>FPTDDDDKIVGGYTCAANSIPYQVSLNSGSHFCGGSLINSQWVVSAAHCYKSRIQVRLGEHNIDVLEGNEQFINAAKIITHPNFNGNTLDNDIMLIKLSSPATLNSRVATVSLPRSCAAAGTECLISGWGNTKSSGSSYPSLLQCLKAPVLSDSSCKSSYPGQITGNMICVGFLEGGKDSCQGDSGGPV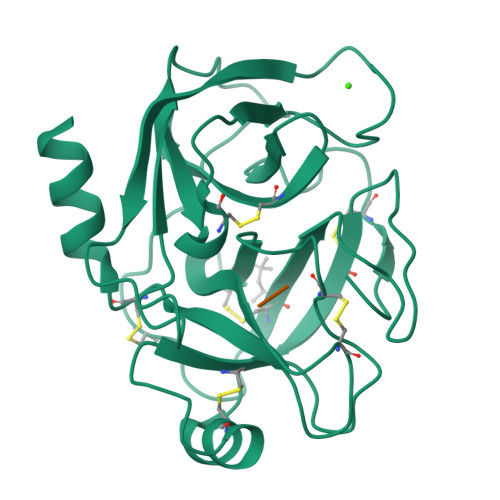VCNGQLQGIVSWGYGCAQKNKPGVYTKVCNYVNWIQQTIAAN[2x]> MDNKLITDLSRVFDYRYVDENEYNFKLISDMLTDFNFSLEYHRNKEVFAHNGEQIKYEHLNVTSSVSDFLTYLNGRFSNMVLGHNGDGINEVKDARVDNTGYDHKTLQDRLYHDYSTLDAFTKKVEKAVDENYKEYRATEYRFEPKEQEPEFITDLSPYTNAVMQSFWVDPRTKIIYMTQARPGNHYMLSRLKPNGQFIDRLLVKNGGHGTHNAYRYIGNELWIYSAVLDANENNKFVRFQYRTGEITYGNEMQDVMPNIFNDRYTSAIYNPIENLMIFRREYKASERQLK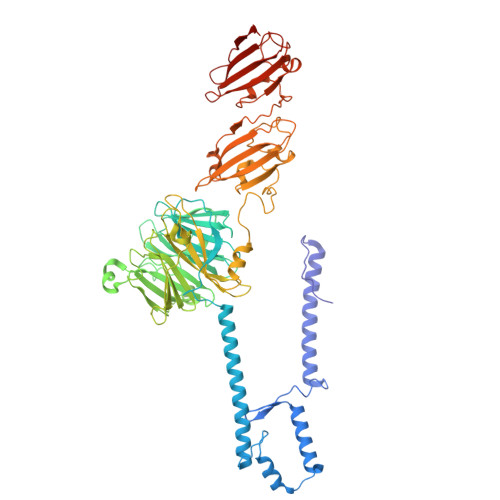NSLNFVEVRSADDIDKGIDKVLYQMDIPMEYTSDTQPMQGITYDAGILYWYTGDSKPANPNYLQGFDIKTKELLFKRRIDIGGVNNNFKGDFQEAEGLDMYYDLETGRKALLIGVTIGPGNNRHHSIYSIGQRGVNQFLKNIAPQVSMTDSGGRVKPLPIQNPAYLSDITEVGHYYIYTQDTQNALDFPLPKAFRDAGWFFDVLPGHYNGALRQVLTRNSTGRNMLKFERVIDIFNKKNNGAWNFCPQNAGYWEHIPKSITKLSDLKIVGLDFYITTEESNRFTDFPKDFKGIAGWILEVKSNTPGNTTQVLRRNNFPSAHQFLVRNFGTGGVGKWSLFEGKVVE N-[4-(acetylamino)butyl]-5'-[(3-{[(4-tert-butylphenyl)carbamoyl]amino}propyl)(propan-2-yl)amino]-5'-deoxyadenosine | 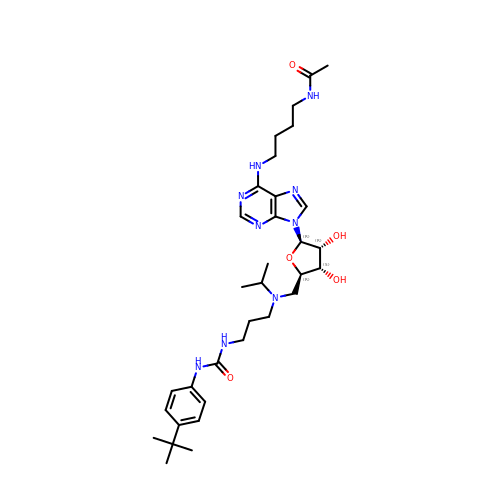C33 H51 N9 O5 | UMDWALJSYFZDHM-QWOIFIOOSA-N>LDRADILYNIRQTSRPDVIPTQRDRPVAVSVSLKFINILEVNEITNEVDVVFWQQTTWSDRTLAWNSSHSPDQVSVPISSLWVPDLAAYNAISKPEVLTPQLARVVSDGEVLYMPSIRQRFSCDVSGVDTESGATCRIKIGSWTHHSREISVDPTTENSDDSEYFSQYSRFEILDVTQKKNSVTYSCC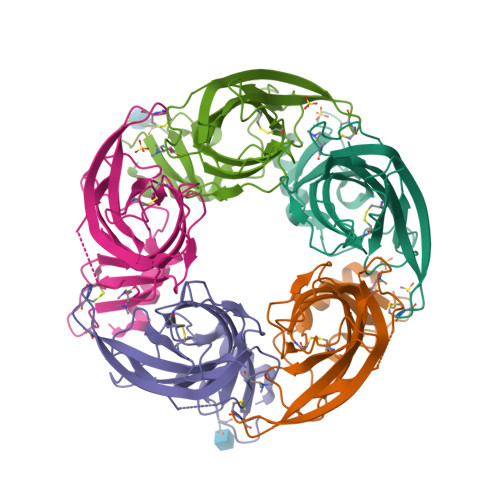PEAYEDVEVSLNFRKKGRSEIL[20x]>MNGDVQSVIRGYLERAQVAKTMSDAGRWNEAGDLLRQLMTDVKSCKISASNRDEHDARNTFLRALEANLKLVQQNVRDEDDLHEAMTRQSGSPEPPADPDVWSKPSPPLPSSSKFGATKKGVGAAGPRPREISKSTSSMSTNPADVKPANPTQGILPQNSAGDSFDASAYDAYIVQAVRGTMATNTENTMSLDDIIGMHDVKQVLHEAVTLPLLVPEFFQGLRSPWKAMVLAGPPGTGKTLIARAIASESSSTFFTVSSTDLSSKWRGDSEKIVRLLFELARFYAPSIIFIDQIDTLGGQRGNSGEHEASRRVKSEFLVQMDGSQNKFDSRRVFVLAATNIPWELDEALRRRFEKRIFIPLPDIDARKKLI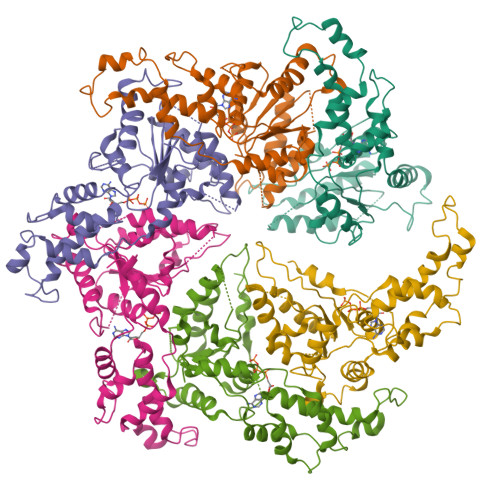EKSMEGTPKSDEINYDDLAARTEGFSGADVVSLCRTAAINVLRRYDTKSLRGGELTAAMESLKAELVRNIDFEAALQAVSPSAGPDTMLKCKEWCDSFGAM[6x]> SMADLSFIEDTVAFPEKEEDEEEEEEGVEWGYEEGVEWGLVFPDANGEYQSPINLNSREARYDPSLLDVRLSPNYVVCRDCEVTNDGHTIQVILKSKSVLSGGPLPQGHEFEL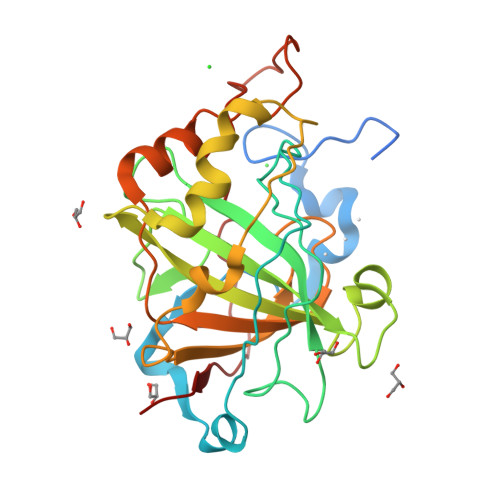YEVRFHWGRENQRGSEHTVNFKAFPMELHLIHWNSTLFGSIDEAVGKPHGIAIIALFVQIGKEHVGLKAVTEILQDIQYKGKSKTIPCFNPNTLLPDPLLRDYWVYEGSLTIPPCSEGVTWILFRYPLTISQLQIEEFRRLRTHVKGAELVEGCDGILGDNFRPTQPLSDRVIRAAFQ>GAMASSNTAATNADSAWLEAQEEEEVGFPVRPQVPLRPMTYKAALDISHFLKEKGGLEGLIWSQRRQEILDLWIYHTQGYFPDWQNYTPGPGIRYPLTFGWCFKLVPVEPEKVEEANEGENNSLLHPMSLHGMEDAEKEVLVWRFDSKLAFHHMARELHPEYY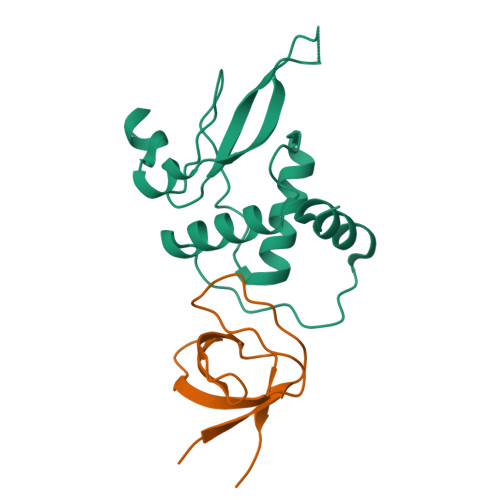KDA[2x];>MEDIIVVALYDYVSWSPDDLSFQKGDQMVVLEESGEWWKARSLATRKEGYIPSNYVARVDS[2x]> MGSDKIHHH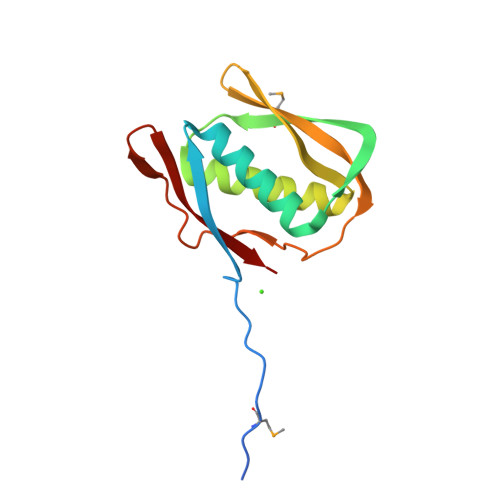HHHMRKPIEHTADIAYEISGNSYEELLEEARNILLEEEGIVLDTEEKEKMYPLEETEDAFFDTVNDWILEISKGWAPWRIKREGNELKVTFRKIRKKEGTEIKALTYHLLKFERDGDVLKTKVVFDT> MKIWLPCDAAAKACGAEAVLAALRLEAEKRGGALDIARNGSRGMIWLEPLLEVETPAGRIGFGPMTPADVPALFDALESHPKALGLVEEIPFFKRQTRLTFARCGRIEPLSLAQFAAAEGWAGLRKALKMTPAEVVEEVLASGLRGRGGAGFPTGIKWRTVAAAQADQKYIVCNVDEGDSGSFADRMLIEGDPFCLVEGMAIAGHAVGATRGYVYIRSEYPDAIAVMRAAIAMAKPFLAEAGFEMEVRVGAGAYVCGEETSLLNSLEGKRGTVRAKPPLPALKGLFGKPTVVNNLLSLAAVPWIIAHGAKAYESFGMDRSRGTIPLQIGGNVKRGGLFETGFGITLGELVEDICGGTASGRPVKAVQVGGPLGAYHPVSDYHLPFCYEQFAGQGGLVGHAGLVVHDDTADMLKLARFAMEFCAIESCGTCTPCRIGAV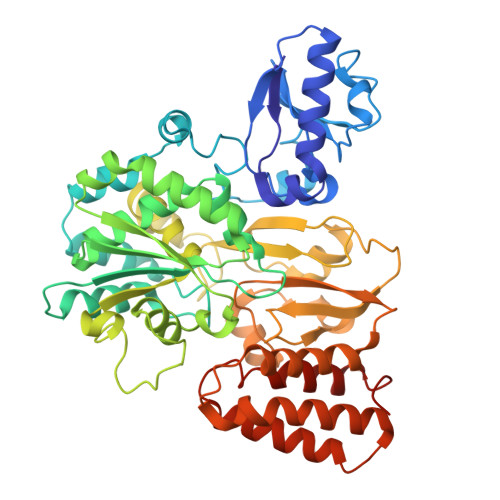RGVEVIDRIAAGDASAMPLLDDLCQTMKLGSLCALGGFTPYPVQSAIRHFPADFPCAREAAE>GAMERVLKVFHYFENSSEPTTWASIIRHGDATDVRGIIQKIVDCHKVKNVACYGLRLSHLQSEEVHWLHLDMGVSNVREKFELAHPPEEWKYELRIRYLPKGFLNQFTEDKPTLNFFYQQVKNDYMLEIADQVDQEIALKLGCLEIRRSYGEMRGNALEKKSNYEVLEKDVGLRRFFPKSLLDSVKAKTLRKLIQQTFRQFANLNREESILKFFEILSPVYRFDKECFKCALGSSWIISVELAIGPEEGISYLTDKGANPTHLADFNQVQTIQYSNSEDKDRKGMLQLKIAGAPEPLTVTAPSLTIAENMADLIDGYCRLVNGATQSFIIRPQKEGERALPSIPKLANNEKQGVR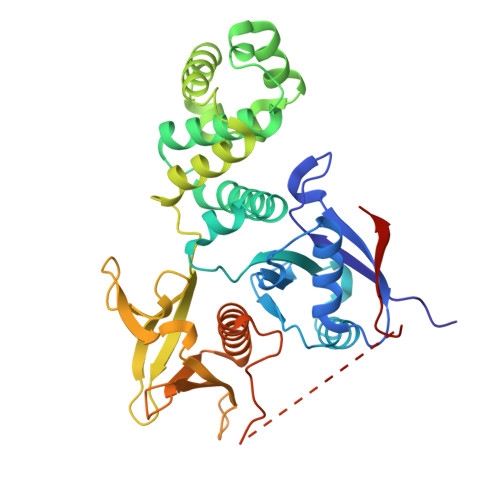SHTVSVSETDDYAEIIDEED[2x]>[2x]MGKKMMTTDGNTATAHVAYAMSEVAAIYPITPSSTMGEEADDWAAQGRKNIFGQTLTIREMQSEAGAAGAVHGALAAGALTTTFTASQGLLLMIPNMYKISGELLPGVFHVTARAIAAHALSIFGDHQDIYAARQTGFAMLASSSVQEAHDMALVAHLAAIESNVPFMHFFDGFRTSHEIQKIEVLDYADMASLVNQKALAEFRAKSMNPEHPHVRGTAQNPDIYFQGREAANPYYLKVPGIVAEYMQKVASLTGRSYKLFDYVGAPDAERVIVSMGSSCETIEEVINHLAAKGEKIGLIKVRLYRPFVSEAFFAALP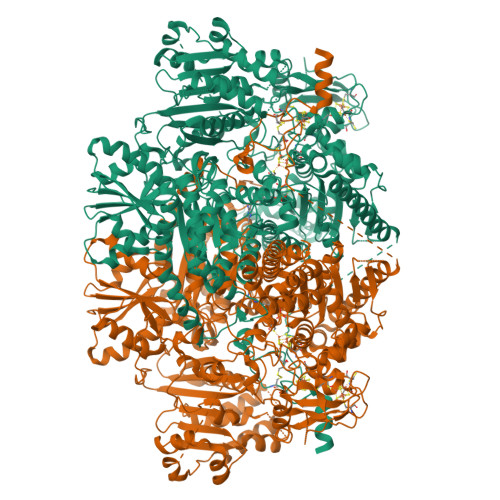ASAKVITVLDRTKEPGAPGDPLYLDVCSAFVERGEAMPKILAGRYGLGSKEFSPAMVKSVYDNMSGAKKNHFTVGIEDDVTGTSLPVDNAFADTTPKGTIQCQFWGLGADGTVGANKQAIKIIGDNTDLFAQGYFSYDSKKSGGITISHLRFGEKPIQSTYLVNRADYVACHNPAYVGIYDILEGIKDGGTFVLNSPWSSLEDMDKHLPSGIKRTIANKKLKFYNIDAVKIATDVGLGGRINMIMQTAFFKLAGVLPFEKAVDLLKKSIHKAYGKKGEKIVKMNTDAVDQAVTSLQEFKYPDSWKDAPAETKAEPMTNEFFKNVVKPILTQQGDKLPVSAFEADGRFPLGTSQFEKRGVAINVPQWVPENCIQCNQCAFVCPHSAILPVLAKEEELVGAPANFTALEAKGKELKGYKFRIQINTLDCMGCGNCADICPPKEKALVMQPLDTQRDAQVPNLEYAARIPVKSEVLPRDSLKGSQFQEPLMEFSGACSGCGETPYVRVITQLFGERMFIANATGCSSIWGASAPSMPYKTNRLGQGPAWGNSLFEDAAEYGFGMNMSMFARRTHLADLAAKALESDASGDVKEALQGWLAGKNDPIKSKEYGDKLKKLLAGQKDGLLGQIAAMSDLYTKKSVWIFGGDGWAYDIGYGGLDHVLASGEDVNVFVMDTEVYSNTGGQSSKATPTGAVAKFAAAGKRTGKKDLARMVMTYGYVYVATVSMGYSKQQFLKVLKEAESFPGPSLVIAYATCINQGLRKGMGKSQDVMNTAVKSGYWPLFRYDPRLAAQGKNPFQLDSKAPDGSVEEFLMAQNRFAVLDRSFPEDAKRLRAQVAHELDVRFKELEHMAATNIFESFAPAGGKADGSVDFGEGAEFCTRDDTPMMARPDSGEACDQNRAGTSEQQGDLSKRTKK> EKIPIIVGDYGPMWVYPTSTFDCVVADPRKGSKMYGLKSYIEYQLTPTNTNRSVNHRYKHFDWLYERLLVKFGSAIPIPSLPDKQVTGRFEEEFIKMRMERLQAWMTRMCRHPVISESEVFQQFLNFRDEKEWKTGKRKAERDELAGVMIFSTMEPEAPDLDLVEIEQKCEAVGKFTKAMDDGVKELLTVGQEHWKRCTGPLPKEYQKIGKALQSLATVFSSSGYQGETDLNDAITEAGKTYEEIASLVAEQPKKDLHFLMECNHEYKGFLGCFPDII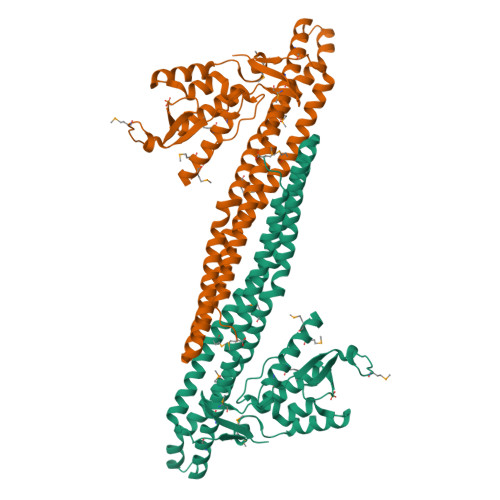GTHKGAIEKVKESDKLVATSKITLQDKQNMVKRVSIMSYALQAEMNHFHSNRIYDYNSVIRLYLEQQVQFYETIAEKLRQALSRFPVM>MLPAPKNLV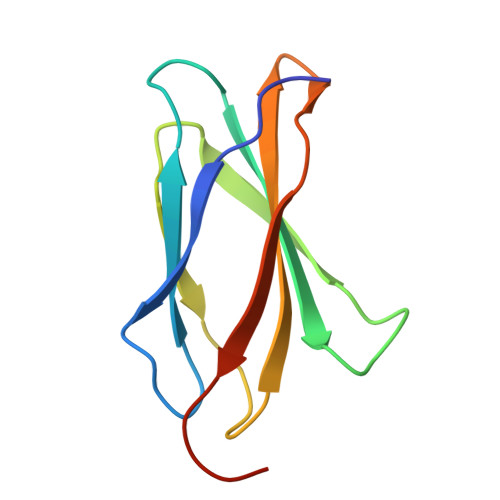VSEVTEDSLRLSWTAPDAAFDSFMIQYQESEKVGEAINLTVPGSERSYDLTGLKPGTEYTVSIYGVKGGHRSNPLSAEFTTGGHHHHHH[4x]(3S)-3-(2-benzyl-3-chloro-7-oxo-2,4,5,7-tetrahydro-6H-pyrazolo[3,4-c]pyridin-6-yl)-5-methyl-4-oxo-2,3,4,5-tetrahydro-1,5-benzoxazepine-8-carbonitrile | C24 H20 Cl N5 O3 | 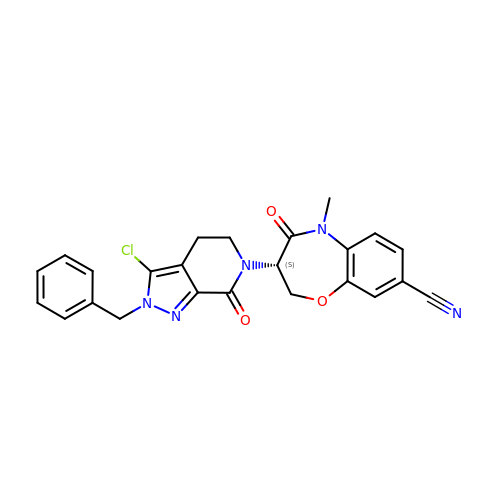JWKONLKXWPCOJF-IBGZPJMESA-N> MDEIDLRILKILQYNAKYSLDEIAREIRIPKSTLSYRIKKLEKDGVIKGYYAYINPASLNLDYIVITSVKAKYGKNYHVELGNKLAQIPGVWGVYFVLGDNDFIVMARYKTREEFMEKFLERVMSIPE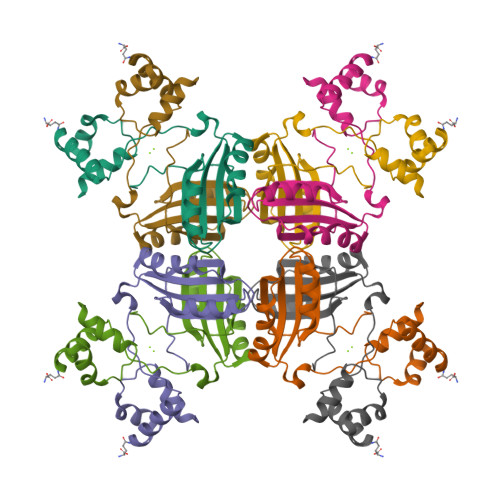VERASTQVVVKIIKESPNIVIF> GD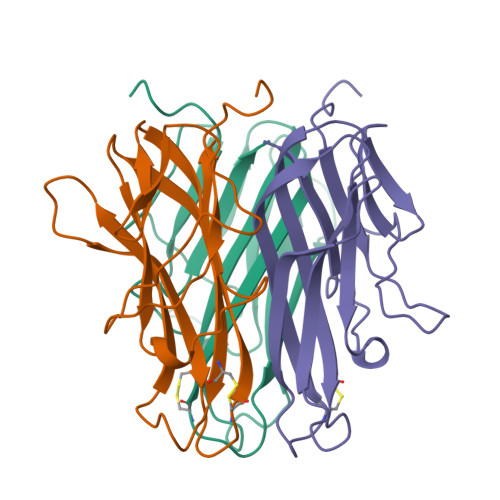QNPQIAAHVISEASSKTTSVLQWAEKGYYTMSNNLVTLENGKQLTVKRQGLYYIYAQVTFCSNREASSQAPFIASLCLKSPGRFERILLRAANTHSSAKPCGQQSIHLGGVFELQPGASVFVNVTDPSQVSHGTGFTSFGLLKL>[4x]GASNEVLVLRGTLEGHNGWVTSLATSAGQPNLLLSASRDKTLISWKLTGDDQKFGVPVRSFKGHSHIVQDCTLTADGAYALSASWDKTLRLWDVATGETYQRFVGHKSDVMSVDIDKKASMIISGSRDKTIKVWTIKGQCLATLLGHNDWVSQVRVVPNEKADDDSVTIISAGNDKMV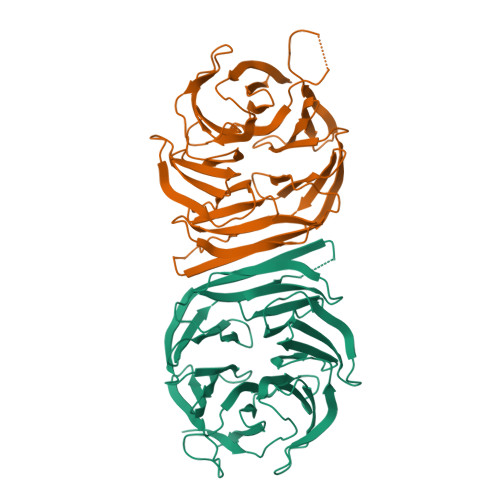KAWNLNQFQIEADFIGHNSNINTLTASPDGTLIASAGKDGEIMLWNLAAKKAMYTLSAQDEVFSLAFSPNRYWLAAATATGIKVFSLDPQYLVDDLRPEFAGYSAAAEPHAVSLAWSADGQTLFAGYTDNVIRVWQVMTAN> VGLTTLFWLGAIGMLVGTLAFAWAGRDAGSGERRYYVTLVGISGIAAVAYVVMALGVGWVPVAERTVFAPRYIDWILTTPLIVYFLGLLAGLDSREFGIVITLNTVVMLAGFAGAMVPGIERYALFGMGAVAFLGLVYYLVGPMTESASQRSSGIKSLYVRLRNLTVILWAIYPFIWLLGPPG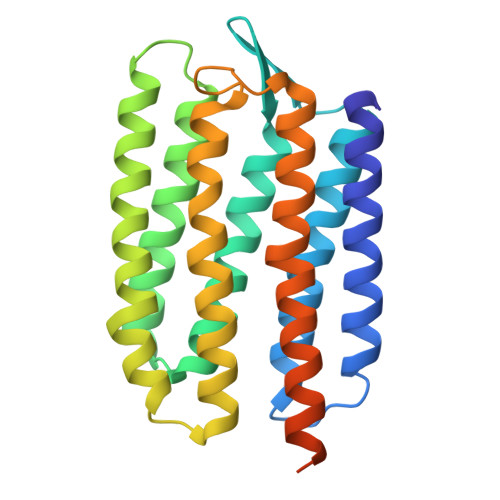VALLTPTVDVALIVYLDLVTKVGFGFIALDAAATLRAEHGESLAGVDTDAPAVADENSHHHHHHH> GPDLTEDWKEALEWMRTSLEEQNYLNPYEKPEYSVMSWWDYGNWILYVSKKAVVANNFQAGAVDA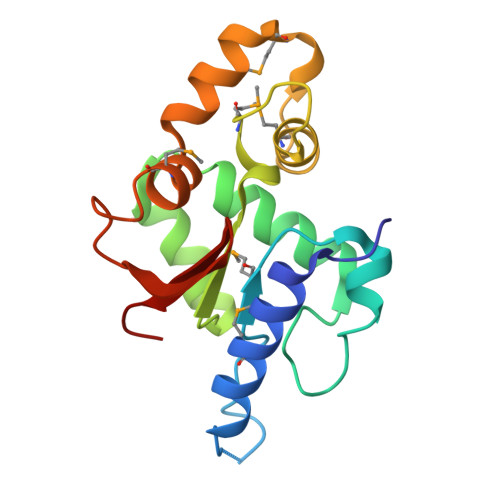AKFFTAKSEDEAIKIAKKRGVRYVVTADEITMKDANNTKFPAIMRIAGYNVDLMTEGEILNFFNHTVLYRLHMENAENLTHFRLVKEFGDVKIFEVVGS~{N}-[(5-methylfuran-2-yl)methyl]-5-thiophen-2-yl-4~{H}-1,2,4-triazol-3-amine 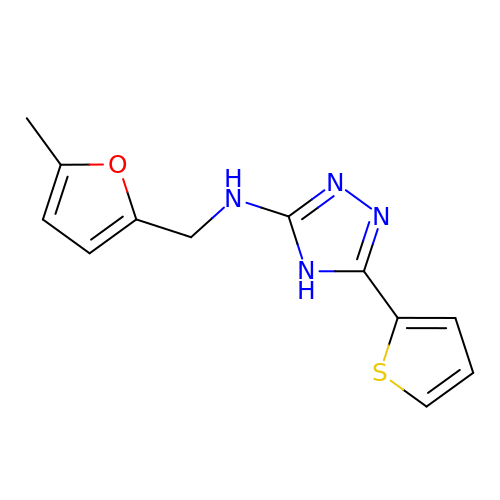| C12 H12 N4 O S | BXCLKGCUMNDSFV-UHFFFAOYSA-N> DHSELLVNTKSGKVMGTRVPVLSSHISAFLGIPFAEPPVGNMRFRRPEPKKPWSGVWNASTYPNNCQQYVDEQFPGFSGSEMWNPNREMSEDCLYLNIWVPSPRPKSTTVMVWIYGGGFYSGSSTLDVYNGKYLAYTEEVVLVSLSYRVGAFGFLALHGSQEAPGNVGLLDQRMALQWVHDNIQFFGGDPKTVTIFGESAGGASVGMHILSPGSRDLFRRAILQSGSPNCPWASVSVAEGRRRAVELGRNLNCNLNSDEELIHCLREKKPQELIDVEWNVLPFDSIFRFSFVPVIDGEFFPTSLESMLNSGNFKKTQILLGVNKDEGSFFLLYGAPGFSKDSESKISREDFMSGVKLSVPHANDLGLDAVTLQYTDWMDDNNGIKNRDGLDDIVGDHNVICPLMHFVNKYTKFGNGTYLYFFNHRASNLVWPEWMGVIHGYEIEFVFGLPLVKELNYTAEEEALSRRIMHYWATFAKTGNPNEPHSQESKWPLFTTKEQKFIDLNTEPMKVHQRLRVQMCVF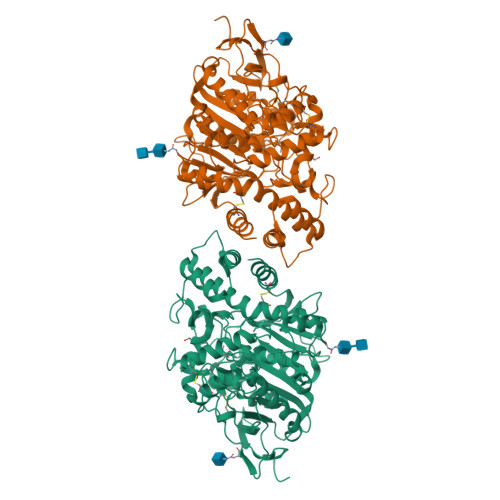WNQFLPKLLNAT>[6x]MEARTTDLSDLYPEGEALPMVFKSFGGRARFAGRVRTLRV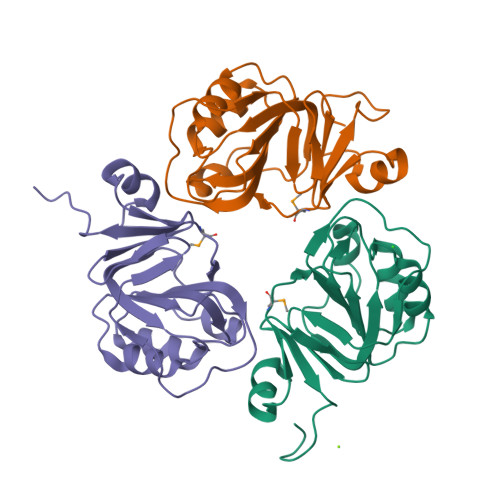FEDNALVRKVLEEEGAGQVLFVDGGGSLRTALLGGNLARRAWEKGWAGVVVHGAVRDTEELREVPIGLLALAATPKKSAKEGKGEVDVPLKVLGVEVLPGSFLLADEDGLLLLPEPPSGVRSGG> TCNIKNGRCEQFCKNSADNKVVCSCTEGYRLAENQK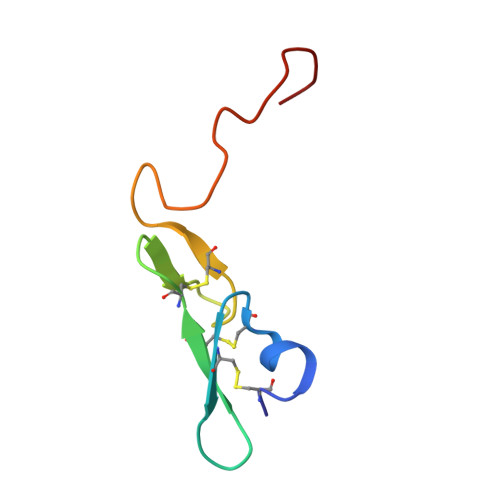SCEPAVPFPCGRVSVSQTSKLTR>[2x]AVSPKTYKDADFYVAPTQQDVNYDLVDDFGANGNDTSDDSNALQRAINAISRKPNGGTLLIPNGTYHFLGIQMKSNVHIRVESDVIIKPTWNGDGKNHRLFEVGVNNIVRNFSFQGLGNGFLVDFKDSRDKNLAVFKLGDVRNYKISNFTIDDNKTIFASILVDVTERNGRLHWSRN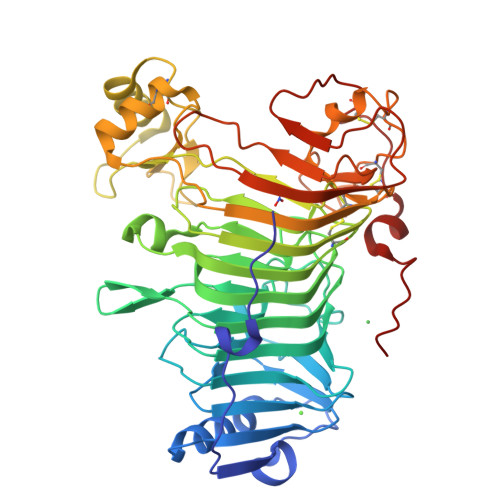GIIERIKQNNALFGYGLIQTYGADNILFRNLHSEGGIALRMETDNLLMKNYKQGGIRNIFADNIRCSKGLAAVMFGPHFMKNGDVQVTNVSSVSCGSAVRSDSGFVELFSPTDEVHTRQSWKQAVESKLGRGCAQTPYARGNGGTRWAARVTQKDACLDKAKLEYGIEPGSFGTVKVFDVTARFGYNADLKQDQLDYFSTSNPMCKRVCLPTKEQWSKQGQIYIGPSLAAVIDTTPETSKYDYDVKTFNVKRINFPVNSHKTIDTNTESSRVCNYYGMSECSSSRWERLEHHHHHH> GSHMSDEVSLYTTREPKLIQPLLDAFAKDSGIKVNTVFVKDGLLERVRAEGDKSPADVLMTVDIGNLIDLVNGGVTQKIQSQTLDSVVPANLRGAEGSWYALSLRDRVLYVEKDLKLDSFRYGDLADP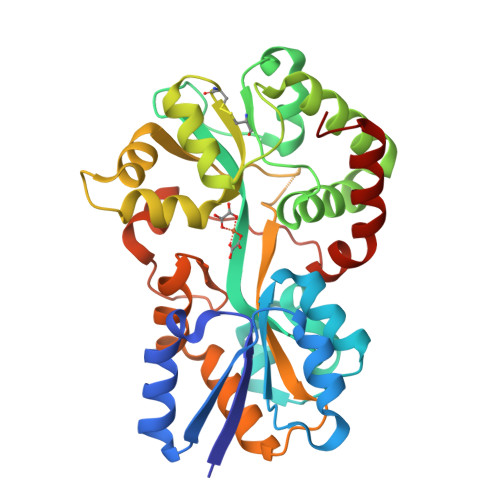KWKGKVCIRSGQHPYNTALVAAMIAHDGAEATEKWLRGVKANLARKAAGGDRDVARDILGGICDIGLANAYYVGHMKNAEPGTDARKWGDAIKVVRPTFATAKDGGTHVNISGAAVAAHAPNKANAVKLLEYLVSEPAQTLYAQANYEYPVRAGVKLDAVVASFGPLKVDTLPVAEIAKYRKQASELVDKVGFDN> VVGGEDAKPGQFPWQVVLNGKVDAFCGGSIVNEKWIVTAAHCVETGVKITVVAGEHNIEETEHTEQKRNVIRIIPHHNYNAAINKYNHDIA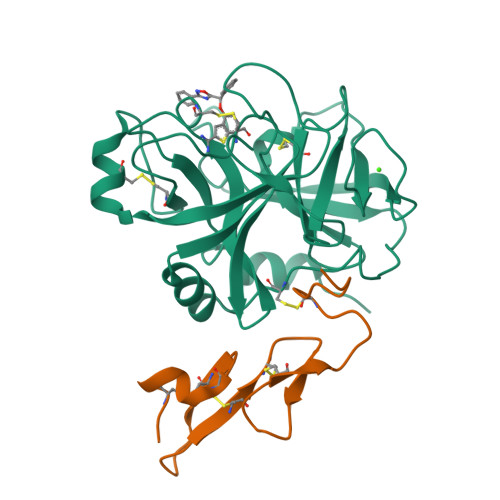LLELDEPLVLNSYVTPICIADKEYTNIFLKFGSGYVSGWGRVFHKGRSALVLQYLRVPLVDRATCLRSTKFTIYNNMFCAGFHEGGRDSCQGDSGGPHVTEVEGTSFLTGIISWGEECAMKGKYGIYTKVSRYVNWIKEKTKLT;> MTCNIKNGRCEQFCKNSADNKVVCSCTEGYRLAENQKSCEPAVPFPCGRVSVSQTSK> SNALRKPLNWDLETFQFTNQDGKPFGTKDLKGKVWVADFMFTNCQTVCPPMTANMAKLQKMAKEEKLDVQFVSFSVDPDLDKPENLKAFIQKFTEDTSNWNLLTGYSLEDITKFSKDNFQSLVDKPENGQVIHGTS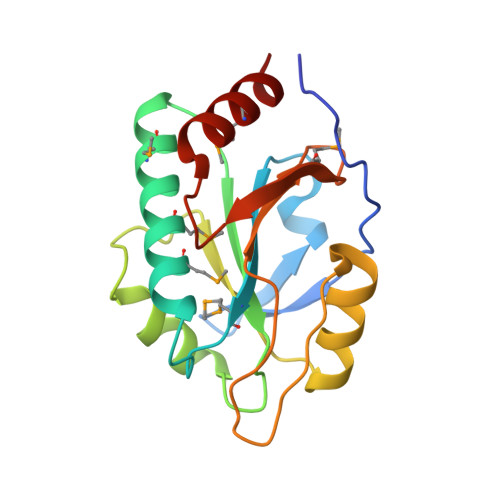FYLIDQNGKVMKKYSGISNTPYEDIIRDMKRLAE> AGKAFKPEELRQALMPTLEALYRQDPESLPFRQPVDPQLLGIPDYFDIVKSPMDLSTIKRKLDTGQYQEPWQYVDDIWLMFNNAWLYNRKTSAVYKYCSKLSEVFEQEIDPVMQSLGYCCGRKLGELFVECTECGRKMHQICVLHHEIIWPAG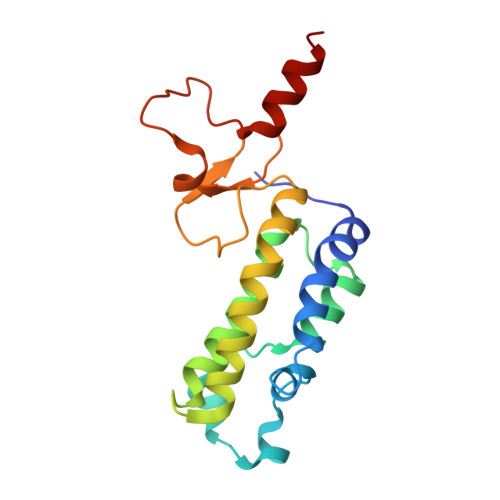FVCDGCLKKSARTRK>[4x]MNRIKTINDHINPRDLSLTEIAKHNTEEDCWVIIKDIVYDLTKFLPDHP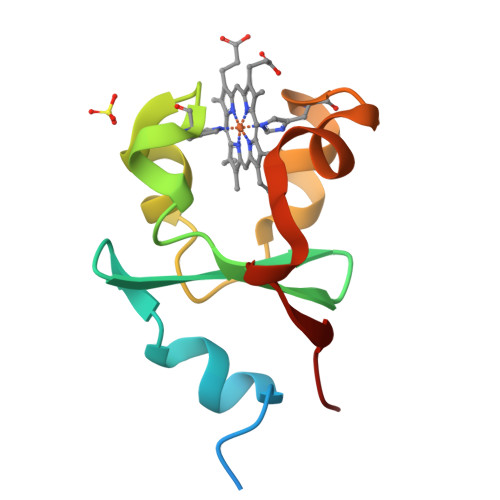GGKKAIILFAGKDATEEFDMLHPPNVLKKYLTPEVVLGPVKK>GPLGSTDLYTDNRTKKKVAHRERKQDFSAFKQTDSEMKVKISPQLLLAMHRFLATEVEAFSPSQMSEKILLRLLKHPNVIQELKYDEKNKKAPEYYLYQRNKPVDYFVLILQGKVEVEAGKEGMKFEASAFSYYGVMALTASPVIDAVTPT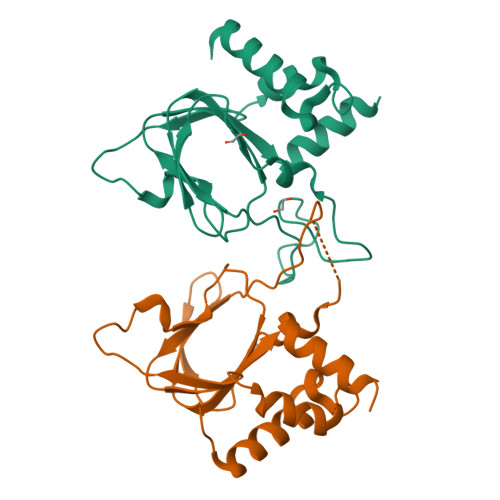LGSSNNQLNSSLLQVYIPDYSVRALSDLQFVKISRQQYQNALMASRMD[2x]> GSTLQPLENSTRQEKLLYPKLNQLSNSINAAVAFLLEAR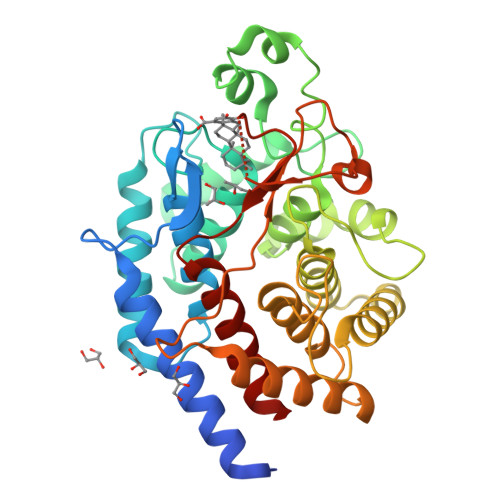NLEGWWQDFNFPQAASIGDEWVTAYVGTMLATLPYAHVHEALMQAWELLKIRDHRPTGEWGYNYILCGDAATTGWALQLAAAVGASDSERAQQARAALATHLQPNGGIATFAEESIRAYIKVPDLANVSFQGWCGAHTCVSAAVAALPEFRSRLHDYLRVTQTSQGNWEGYWWSDHEYTTALTAEALAAGGQAADQPSIEQAVAWGLKRLCPQGFVATSKHPNGSTFATAWCLRLLLLNTVDAEVKAARAAAIGWLLEQQRPNGSWVSSAYLRIPYPFDRNPNQFPHWRYYDEIEGDKRFEGSIIFDHNSIFTTATVVNSLVKAAPML>QDSTSDLIPAPPLSKVPLQQNFQDNQFHGKWYQVG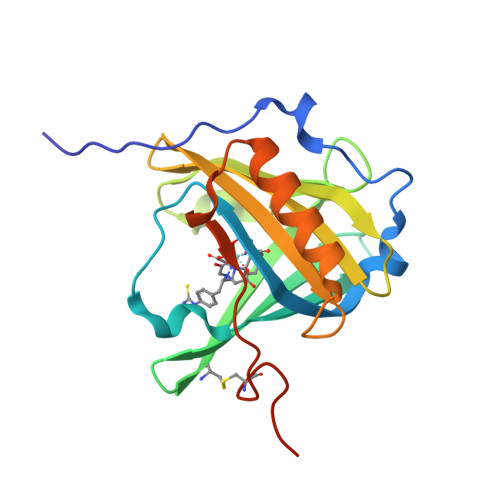RAGNAAPREDKDLLKMTAQTYELKEDKSYNVTAVRFRKKMCEYLTMTFVPGSQPGEFTLGNIKSYPGLTSYLVRVVSTNYNQHAMVFFKKVQQNREYFSISLLGRTKELASELKENFIRFSKSLGLPENHIVFPVPIDQCIDGSAWSHPQFEK[3x]> MFHLVDFQ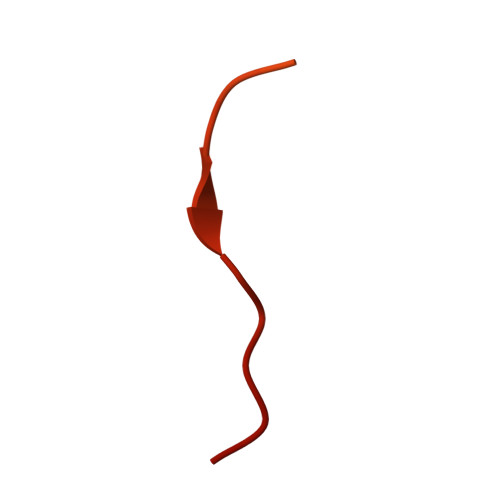VTIAEILIIIMRTFRIAIWNLDVIISSIVRQLFKPLTKKNYSELDDEEPMELDYP> MEHIRTTKVEQVKLLDRFSTSNKSLTGTLYLTATHLLFIDSHQKETWILHHHIASVEKLALTTSGCPLVIQCKNFRTVHFIVPRERDCHDIYNSLLQL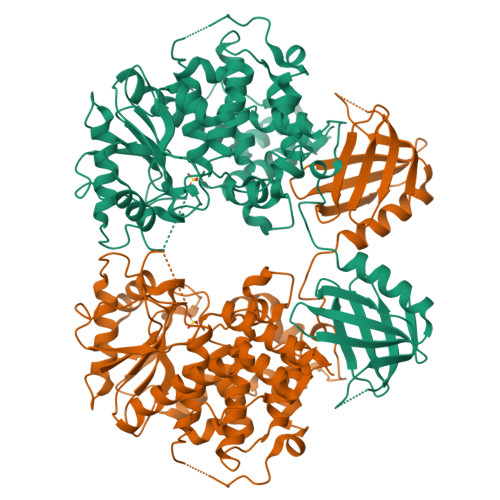SKQAKYEDLYAFSYNPKQNDSERLQGWQLIDLAEEYKRMGVPNSHWQLSDANRDYKICETYPRELYVPRIASKPIIVGSSKFRSKGRFPVLSYYHQDKEAAICRCSQPLSGFSARCLEDEHLLQAISKANPVNRYMYVMDTRPKLNAMANRAAGKGYENEDNYSNIRFQFVGIENIHVMRSSLQKLLEVNGTKGLSVNDFYSGLESSGWLRHIKAVMDAAVFLAKAITVENASVLVHCSDGWDRTSQVCSLGSLLLDSYYRTIKGFMVLIEKDWISFGHKFSERCGQLDGDPKEVSPVFTQFLECVWHLTEQFPQAFEFSEAFLLQIHEHIHSCQFGNFLGNCQKEREELKLKEKTYSLWPFLLEDQKKYLNPLYSSESHRFTVLEPNTVSFNFKFWRNMYHQFDRTAHHHHHH> MAPVPEPEVVATPPADAGRGLIRVDSREIRHYSGTRKEPDYLVSRDNGKTWEMKAAPAGYPPNYGGIPKESPAIVRNPLTREFIRVQPIGGFVFLSRGGLDGKWLAVTNDGKLEEDWKDPEKRKNLKKLGGIMRTPVFVNKGRRVIVPFHNMGGGTKFHISDDGGLTWHVSRNGVTSPRHEARPPHQGVRWFNNAVEA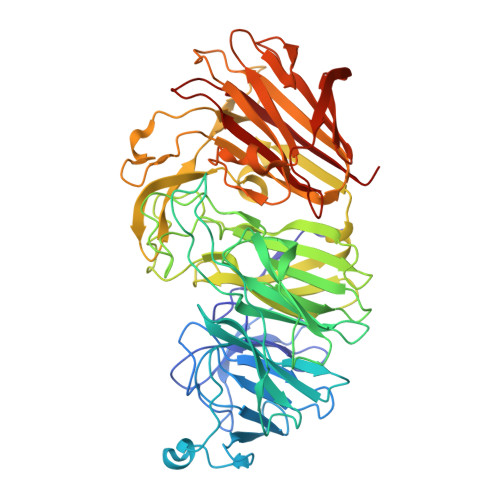TVLEMKDGTLWALARTSQDQAWQAFSKDYGETWSKPEPSRFFGTLTMNTLGRLDDGTIVSLWTNTMALPENATAGNGTWEDVFTNRDSHHIAMSGDEGKTWYGFREIILDEHRNHPGYATLDGPEDRGKHQSEMVQLDKNRILISLGQHKNHRRLVIVDRRWVGAKTRATQTGKDLDSQWTIHTYIPQKKGHCSYNRKPSAELVQDPSGGTKKVLQIKRLDDPELVNEKSNVDYRNGGATWNFPNGTTGLVKFRFRVVDGEQADDSGLQVSLTDRLFNACDSTTKDYALFTFPIRLKPAPHLLLGMKKVPFTPGAWHEISLLWQGGQAVVSLDGKKAGTLKMANKSPNGASYIHFISTGSQPDAGILLDTVNARVKAE>MEAEQVWKLWRRVLRDERLQAQLFSATDATHWLSGFSESESKILSVYAQQFDRVKWFVENYQFRLVNSFLNALETGAPLSLRALLHINVDLNAQSKAFLRDRQWRDYGPQVYTYCEDVLGFLAEADELQGYPEILDLMRLERESVRLYRGLVDPESLPADNRYQRTSMARLYETRFALSGWLRQKDQLGLTRLPESTEHVLIYLPTLQARHKFTLINAQAARLYNCLEQPQSAAGLFMLINSDSASVPGSADLALLDRLEQLNAIRKPL[2x];>MPDFVKPAPIGVGIQYNPEILDWFPFEDIQVDILEILLDNIMAPMDGPQIIKPSAQAMIERLGQKFTLLAHSNYGCDFGFSALEETAAVQRHVPLAKMLNSPWVANHCFYGDQSWLDIWSSPIQFSAAEVARCADRAQSLQTLYGMPLAHENAAYYLECPGAEMREAEFLARLVQRSGTFLHLDLHNIYTNHLNLKGFDLKDYMDTLPLDKVISVHLAGGSWHGGLYHDWHDACVPEPVW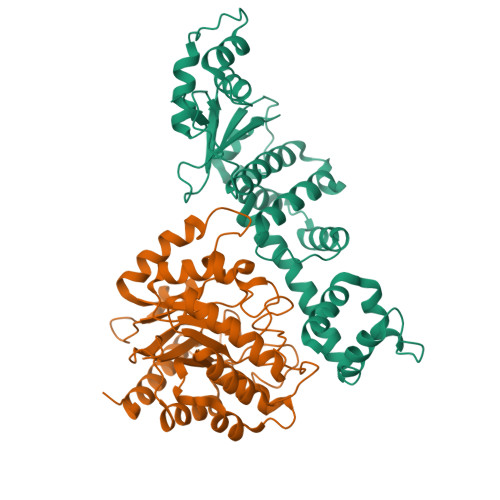DLYEDLLSRAQPSAVILEYQGQAHHAQTRIMDASDESMIVRDVQRAQAIWSRYNRHPQERQYGS[2x]>[2x]MAELCPLAEELSCSICLEPFKEPVTTPCGHNFCGSCLNETWAVQGSPYLCPQCRAVYQARPQLHKNTVLCNVVEQFLQADLAREPPADVWTPPARASAPSPNAQVACDHCLKEAAVKTCLVCMASFCQEHLQPHFDSPAFQDHPLQPPVRDLLRRKCSQHNRLREFFCPEHSECICHICLVEHKTCSPASLSQASADLEATLRHKLTVMYSQINGASRALDDVRNRQQDVRMTANRKVEQLQQEYTEMKALLDASETTSTRKIKEEEKRVNSQFDTIYQILLKKKSEIQTLKEEIEQSLTKR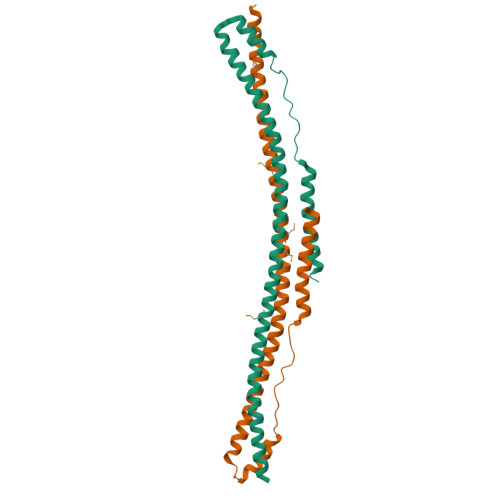DEFEFLEKASKLRGISTQPVYIPEVELNHKLIKGIHQSTIDLKNELKQCIGRLQEPTPSSGDPGEHDPASTHKSTRPVKKVSKEEKKSKKPPPVPALPSKLPTFGAPEQLVDLKQAGLEAAAKATSSHPNSTSLKAKVLETFLAKSRPELLEYYIKVILDYNTAHNKVALSECYTVASVAEMPQNYRPHPQRFTYCSQVLGLHCYKKGIHYWEVELQKNNFCGVGICYGSMNRQGPESRLGRNSASWCVEWFNTKISAWHNNVEKTLPSTKATRVGVLLNCDHGFVIFFAVADKVHLMYKFRVDFTEALYPAFWVFSAGATLSICSPK> MNLIPTVIETTNRGERAYDIYSRLLKDRIIMLGSQIDDNVANSIVSQLLFLQAQDSEKDIYLYINSPGGSVTAGFAIYDTIQHIKPDVQTICIGMAASMGSFLLAAGAKGKRFALPNAEVMIHQPLGGAQGQATEIEIAANHILKTREKLNRILSERTG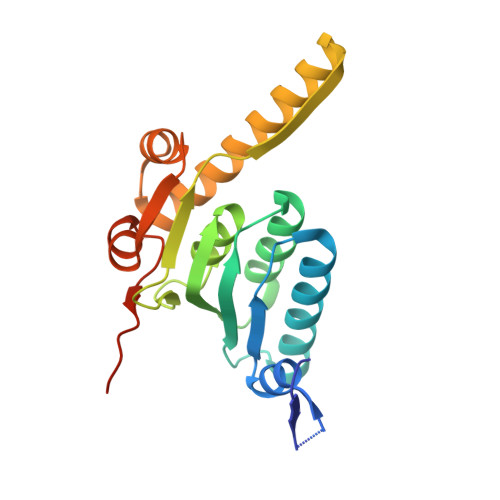QSIEKIQKDTDRDNFLTAEEAKEYGLIDEVMVPETKLEHHHHHH> GLGQMGSSSTDNTVRETVGAATSRDALPNTEASGPTHSKEIPALTAVETGATNPLVPSDTVQTRHVVQHRSRSESSIESFFARGACVTIMTVDNPASTTNKDKLFAVWKITYKDTVQLRRKLEFFTYSRFDMELTFVVTANFTETNNGHALNQVYQIMYVPPGAPVPEKWDDYTWQTSSNPSIFYTYGTAPARISVPYVGISNAYSHFYDGFSKVPLKDQSAALGDSLYGAASLNDFGILAVRVVNDHNPTKVTSKIRVYLKPKHIRVWCPRPPRAVAYYGPGVDYKDGTLTPLSTKDLTTY;> SPNIEACGYSDRVLQLTLGNSTITTQEAANSVVAYGRWPEYLRDSEANPVDQPTEPDVAACRFYTLDTVSWTKESRGWWWKLPDALRDMGLFGQNMYYHYLGRSGYTVHVQCNASKFHQGALGVFAV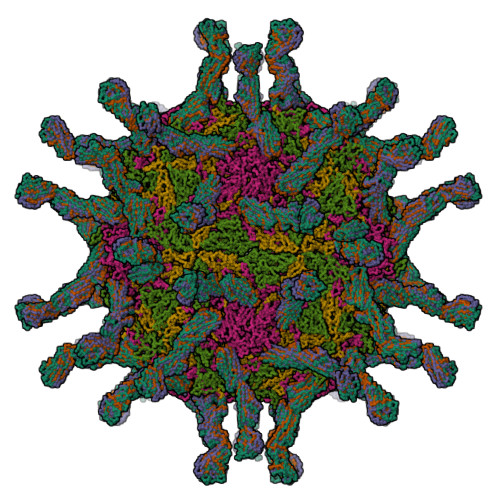PEMCLAGDSNTTTMHTSYQNANPGEKGGTFTGTFTPDNNQTSPARRFCPVDYLLGNGTLLGNAFVFPHQIINLRTNNCATLVLPYVNSLSIDSMVKHNNWGIAILPLAPLNFASESSPEIPITLTIAPMCCEFNGLRNITLPRLQ;> GLPVMNTPGSNQYLTADNFQSPCALPEFDVTPPIDIPGEVKNMMELAEIDTMIPFDLSATKKNTMEMYRVRLSDKPHTDDPILCLSLSPASDPRLSHTMLGEILNYYTHWAGSLKFTFLFCGSMMATGKLLVSYAPPGADPPKKRKEAMLGTHVIWDIGLQSSCTMVVPWISNTTYRQTIDDSFTEGGYISVFYQTRIVVPLSTPREMDILGFVSACNDFSVRLLRDTTHIEQKA;> GAQVSSQKVGAHENSNRAYGGSTINYTTINYYRDSASNAASKQDFSQDPSKFTEPIKDVLIKTAPMLN;>[3x]DVVVQAPTQVPGFLGDSVTLPCYLQVPNMEVTHVSQLTWARHGESGSMAVFHQTQGPSYSESKRLEFVAARLGAELRNASLRMFGLRVEDEGNYTCLFVTFPQGSRSVDIWLRVLAKPQNTAEVQKVQLTGEPVPMARCVSTGGRPPAQITWHSDLGGMPNTSQVPGFLSGTVTVTSLWILVPSSQVDGKNVTCKVEHESFEKPQLLTVNLTVYYPPEVSISGYDNNWYLGQNEATLTCDARSNPEPTGYNWSTTMGPLPPFAVAQGAQLLIRPVDKPINTTLICNVTNALGARQAELTVQV>[6x]MSKKLLFQFDTDATPSVFDVVVGYDGGADHITGYGNVTPDNVGAYVDGTIYTRGGKEKQSTAIFVGGGDMAAGERVFEAVKKRFFGPFRVSCMLDSNGSNTTAAAGVALVVKAAGGSVKGKKAVVLAGTGPVGMRSAALLAGEGAEVVLCGRKLDKAQAAADS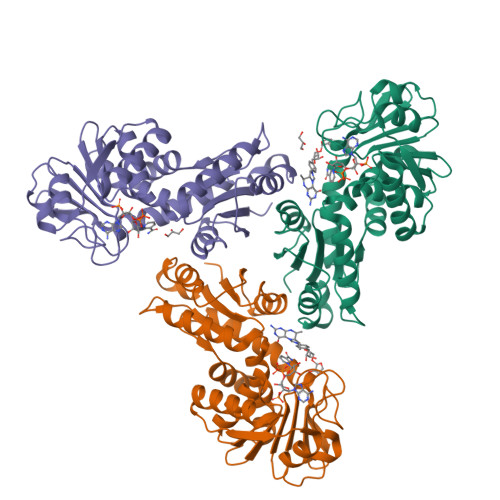VNKRFKVNVTAAETADDASRAEAVKGAHFVFTAGAIGLELLPQAAWQNESSIEIVADYNAQPPLGIGGIDATDKGKEYGGKRAFGALGIGGLKLKLHRACIAKLFESSEGVFDAEEIYKLAKEMAVDKLAAALEHHHHHH[(1S)-1-(5-CHLORO-1-BENZOTHIEN-3-YL)-2-(2-NAPHTHYLAMINO)-2-OXOETHYL]PHOSPHONIC 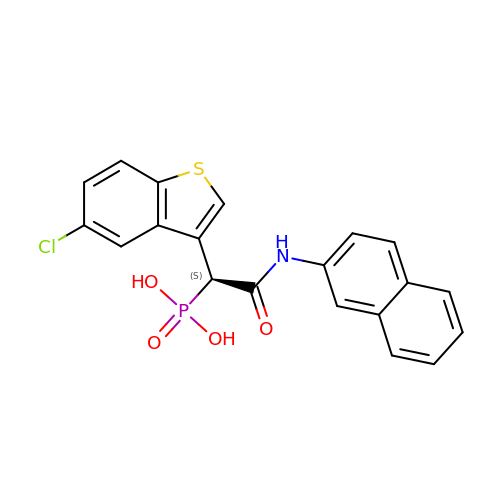ACID | C20 H15 Cl N O4 P S | HUJXISJLAPAFBO-IBGZPJMESA-N Tulane virus (TV) has emerged as a crucial surrogate for HuNoVs due to its close resemblance in amino acid composition and the availability of a robust cell culture system. The structure of TV reveals the characteristic T = 3 icosahedral lattice comprising 90 dimers of the capsid protein VP1. VP1 subunits further divide into two domains: the shell domain (S domain), constituting the inner spherical shell of the virus capsid, and the protruding domain (P domain), further divided into the P1 and P2 sub-domains. In this study, we introduce, through cryo-electron microscopy (cryo-EM), the structure of a specific TV variant (the 9-6-17 TV) that has notably lost its ability to bind to its receptor, B-type HBGA—a finding confirmed using an enzyme-linked immunosorbent assay (ELISA).

To investigate the structural variation in the 9-6-TV, we collected three cryo-EM datasets of the purified 9-6-17 TV. The first dataset that we collected for 9-6-17 TV has inverted image contrast whereby the virus particle is brighter than the background. We reasoned that this was likely caused by the residue iodixanol (OptiPrep) in the buffer not being fully dialyzed away. Despite the reverse contrast, the reconstruction was performed as normal, and the map contrast can be easily inverted by multiplying −1 with the map voxel values. In the end, a 3.2 Å resolution map was generated and the atomic model was derived from it. When we examined the density map of the 9-6-17 TV, we found a density bridge connecting the two subunits of A/B and C/C dimers at the position of Cys452. This density is consistent with the Cys452-Cys452 disulfide bond within all the dimers. A band at around a 120 kDa molecular weight, the mass of a VP1 dimer, was observed in the sample without DTT but not in the sample with DTT. This indicates that the Cys452-Cys452 disulfide bond covalently linked the A/B or C/C subunits in a dimer. Additionally, two mutations (I451M and R452C) are positioned at the interface of the P dimer, contributing to the stabilization of the P dimer through the formation of a disulfide bond. As confirmed by the results of ELISA, it has lost its binding to the original TV host cell receptor, B-type HBGA.

>MESSKTEQVTGATGITQSTVTAPLPEAVSSLSLAPTVNALDPWVYLNQTEVPGGTFTVSSATQPGSVLLELEISPELNLYTSHLFRMYAGWSGGFSLKLLVAGNAFSAGKLIAAIIPPNIEVPNSAYLLTGFPHEILDFRTADSMEIIAPDIKNIDYHFRGDKLGKLVVMVYSPLRSTSADFEIEIKLTSAPLPDFKFTMLVPPIQNNALPIWSIPQAPPYSMVNPRSPLTPVVELYINSSYATCNHQLGRYTIYQGAIGNSTFNPSGAWTATCTAEAGSVTGHPNWRYALLDLPDNPTFDPTLPPVPRGFCDWGSGVKSGNKQHLVCFTGKKVEGGFQDVDTHMWDYGDNETVGLDNTYQRTIYIKDPSLEKDAQYLVIPMGVSGAANDDTVQVAPNCYGSWDYAPTVAPPLGEQFVWFRSQLPASKTTTTSGVNSVPVNVNALMSPDLMCSAYASGFPLGKVALLDYVLFGGSVVRQFKLYPEGYMTANTTGSNTGFIIPADGYFRFNSWVSPSFMISSVVDLNLQTAVVFR[3x]>[2x]EHTWPD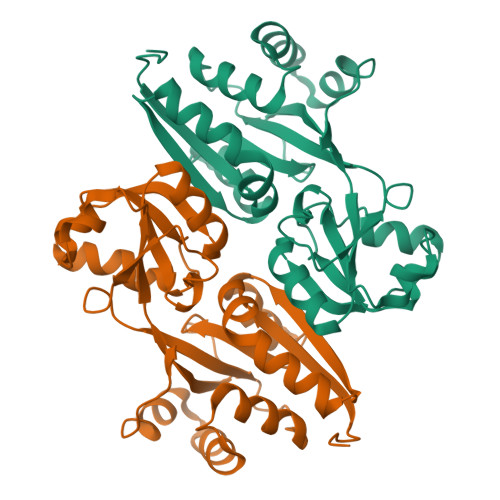KGSLYIATTHTQARYALPGVIKGFIERYPRVSLHMHQGSPTQIAEAVSKGNADFAIATEALHLYDDLVMLPCYHWNRSIVVTPDHPLAATSSVTIEALAQYPLVTYTFGFTGRSELDTAFNRAGLTPRIVFTATDADVIKTYVRLGLGVGVIASMAVDPLADPDLVRIDAHDIFSHSTTKIGFRRSTFLRSYMYDFIQRFAPHLTRDVVDTAVALRSNEEIEAMFQDIKLPEK> MFDFDGYMLRKAKSVNKALEAAVQMKEPLKIHESMRYSLLAGGKRVRPMLCIAACELVGGDESTAMPAACAVEMIHTMSLMHDDLPCMDNDDLRRGKPTNHMAFGESVAVLAGDALLSFAFEHVAAATKGAPPERIVRVLGELAVSIGSEGLVAGQVVDVCSEGMAEVGLDHLEFIHHHKTAALLQGSVVLGAILGGGKEEEVAKLRKFANCIGLLFQVVDDILDVTKS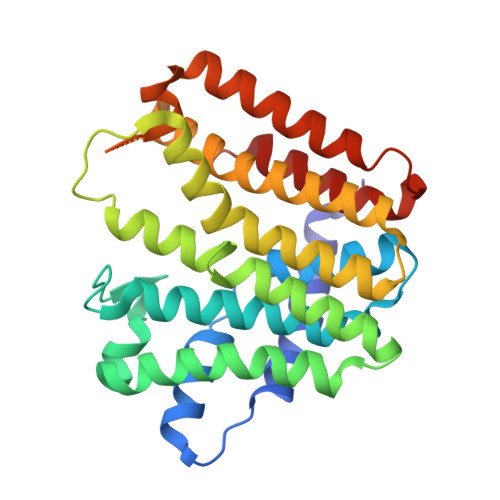SKELGKTAGKDLVADKTTYPKLIGVEKSKEFADRLNREAQEQLLHFHPHRAAPLIALANYIAYRDN> MDWVIPPISLPENEKGPFPKNLVQIKSNKDKEGKVFYSITGQGADTP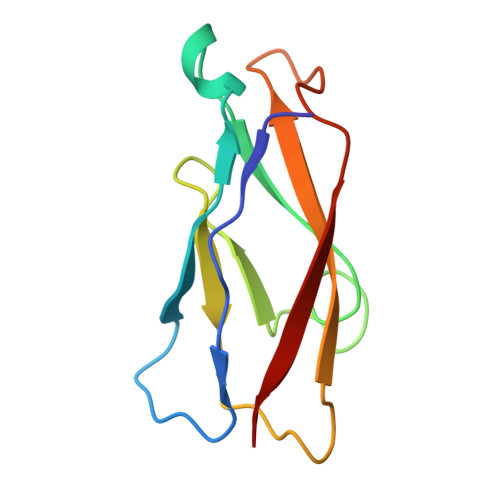PVGVFIIERETGWLKVTEPLDRERIATYTLFSHAVSSNGNAVEDPMEILITVTD> ETGEVTLLDSRSVQGELGWIASPLEGGWEEVSIMDEKNTPIRTYQVCNVMEPSQNNWLRTDWITREGAQRVYIEIKFTLRDCNSLPGVMGTCKETFNLYYYESDNDKERFI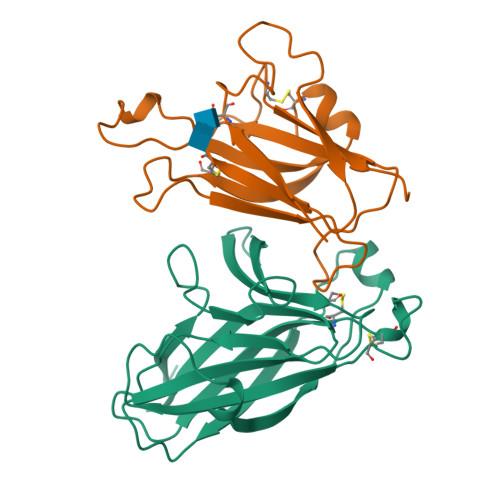RENQFVKIDTIAADESFTQVDIGDRIMKLNTEIRDVGPLSKKGFYLAFQDVGACIALVSVRVFYKRTKHHHHHH;> ETGNSDRYAVYWNRSNPRFHAGAGDDGGGYTVEVSINDYLDIYCPHYGAPLPPAERMEHYVLYMVNGEGHASCDHRQRGFKRWECNRPAAPGGPLKFSEKFQLFTPFSLGFEFRPGHEYYYISATPPNAVDRPCLRLKVYVRPTQETLGTKHHHHHH N-benzoyl-1-[(2R)-3-cyclopentyl-2-{[formyl(hydroxy)amino]methyl}propanoyl]-L-prolinamide 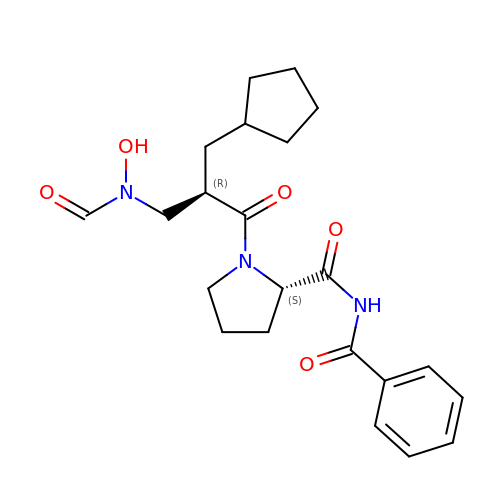| C22 H29 N3 O5 | JPSWIPZHYDYDLN-MOPGFXCFSA-N> IFPKQYPIINFTTADATVESYTNFIRAVRSHLTTGADVRHEIPVLPNRVGLPISQRFILVELSNHAELSVTLALDVTNAYVVGCRAGNSAYFFHPDNQEDAEAITHLFTDVQNSFTFAFGG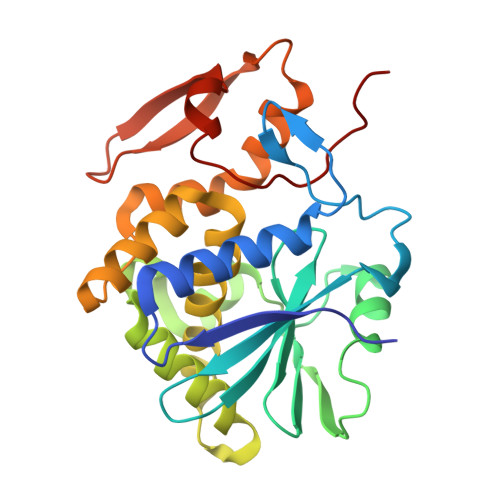NYDRLEQLGGLRENIELGTGPLEDAISALYYYSTCGTQIPTLARSFMVCIQMISEAARFQYIEGEMRTRIRYNRRSAPDPSVITLENSWGRLSTAIQESNQGAFASPIQLQRRNGSKFNVYDVSILIPIIALMVYRCAPPP(2S)-3-{[(3R,7S,11S,15S)-3,7,11,15,19-pentamethylicosyl]oxy}-2-{[(2R,6S,10S,14R)-2,6,10,14,18-pentamethylnonadecyl]oxy}propyl dihydrogen 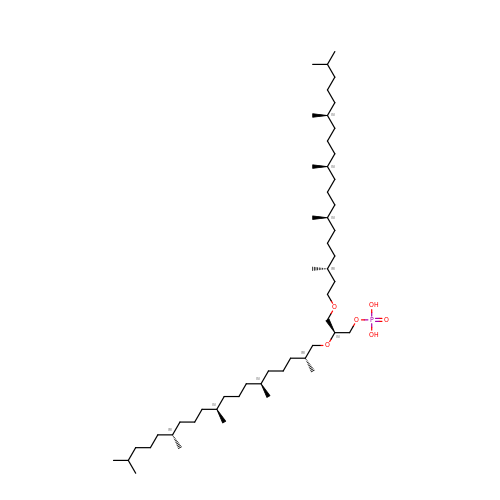phosphate | C52 H107 O6 P | LOOIOWMHQRRBDQ-UYUJORPFSA-N> GSHMLRLSAPGQLDDDLCLLGDVQVPVFLLRLGEASWALVEGGISRDAELVWADLCRWVADPSQVHYWLITHKHYDHCGLLPYLCPRLPNVQVLASERTCQAWKSESAVRVVERLNRQLLRAEQRLPEACAWDALPVRAVADGEWLELGPRHRLQVIEAHGHSDDHVVFYDVRRRRLFCGDALGEFDEAEGVWRPLVFDDMEAYLESLERLQRLPTLLQLIPGHGGLLRGR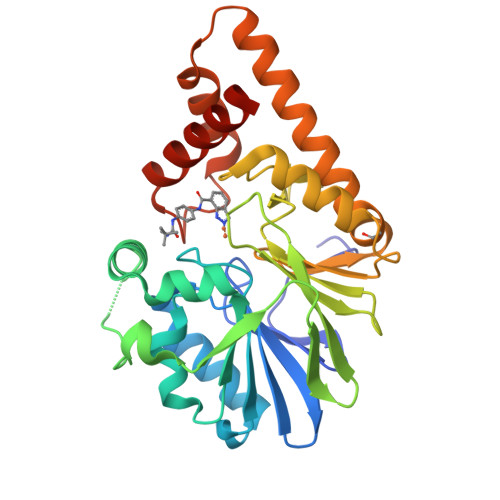LAADGAESAYTECLRLCRRLLWRQSMGESLDELSEELHRAWGGQSVDFLPGELHLGSMRRMLEILSRQALPLD>[2x]MPQYQTWEEFSRAAEKLYLADPMKARVVLKYRHSDGNLCVKVTDDLVCL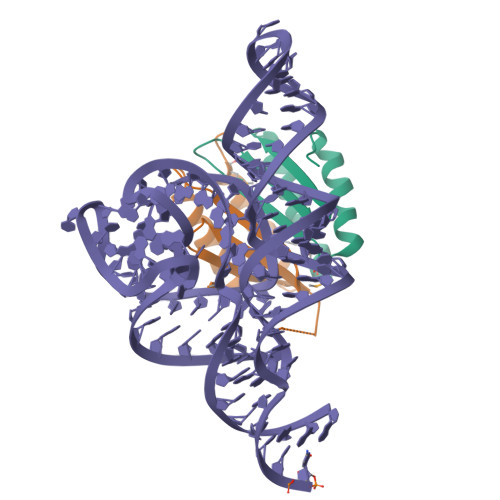VYKTDQAQDVKKIEKFHSQLMRLMVAKEARNVTMET;>[2x]MVLLESEQFLTELTRLFQKCRTSGSVYITLKKYDGRTKPIPKKGTVEGFEPADNKCLLRATDGKKKISTVVSSKEVNKFQMAYSNLLRANMDGLKKRDKKNKTKKTK>[7x]AYTKISDVIVPELFNPYVINTTTQLSAFFQSGIAATDDELNALAKKAGGGSTLNMPYWNDLDGDSQVLNDTDDLVPQKINAGQDKAVLILRGNAWSSHDLAATLSGSDPMQAIGSRVAAYWAREMQKIVFAELAGVFSNDDMKDNKLDISGTADGIYSAETFVDASYKLGDHESLLTAIGMHSATMASAVKQDLIEFVKDSQSGIRFPTYMNKRVIVDDSMPVETLEDGTKVFTSYLFGAGALGYAEGQPEVPTETARNALGSQDILINRKHFVLHPRGVKFTENAMAGTTPTDEELANGANWQRVYDPKKIRIVQFKHRLQA

Here we report near-atomic models built into cryo-EM structures of procapsid I, intermediate procapsid II which has partially released the SP, and the mature DNA-filled capsid from bacteriophage SPP1. The structures are T = 7 laevo icosahedra composed of 415 copies of the MCP gp13 (35.4 kDa), several hundred copies of SP gp11 (23.5 kDa) inside procapsids, 180 copies of gp12 in DNA-filled capsids, and a gp6-gp7 complex which forms the specialised portal vertex. The asymmetric units (ASUs) comprise seven SPP1 gp13 subunits: six in a hexon (subunits A to F) and one from the capsid penton (subunit G). Gp13 has the characteristic L-shape of capsid proteins of other tailed bacteriophages, with well-defined A and P domains, an extended N-terminus arm, and the E-loop.

The mature virion capsid (MVC) packed with DNA was reconstructed from images of the infectious SPP1 phage particles. The MVC has the same size and protein shell thickness as procapsid II. The capsid is filled with densely packed dsDNA appearing as concentric layers of density. The opening is closed in the MVC state whose hexon is nearly flat and only 1 nm longer than in procapsid II. The overall fold of the 324 amino acids-long SPP1 gp13 in the MVC is similar to gp5 in the mature empty capsid of phage HK977 in spite of only 12% sequence identity. During transition from procapsid II to the post-DNA packaging capsid state (MVC) hairpin β6–β7 of the hexons unfolds to form the A-loop, which turns outwards closing the hexon central opening. Subunits A to E remain nearly unchanged during transition from procapsid II to the MVC. In contrast, subunits F and G undergo a significant structural rearrangement similar to the transition of subunits A–E from procapsid I to procapsid II when the SP is released. Gp12 binds to a ring of six Glu197 that converge from the tip of the A loop closing the hexamer central hole. The major structural change found in hexons of the mature capsids is the outward motion of the A loops, probably caused by DNA packaging inside the capsid, closing the central openings and creating the binding site for the gp12 trimeric auxiliary protein.>MGKTYYDNNNSANYQVSTHMASIPSSASVQLDSYNYDGSTFSGKIYVKNIAYSKKVTVVYADGSDNWNNNGNIIAASFSGPISGSNYEYWTFSASVKGIKE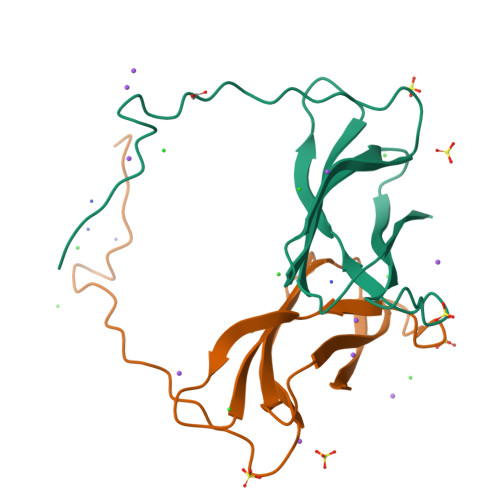FYIKYEVS[2x]(R)-3-CARBOXY-2-(HEXANOYLOXY)-N,N,N-TRIMETHYLPROPAN-1-AMINIUM 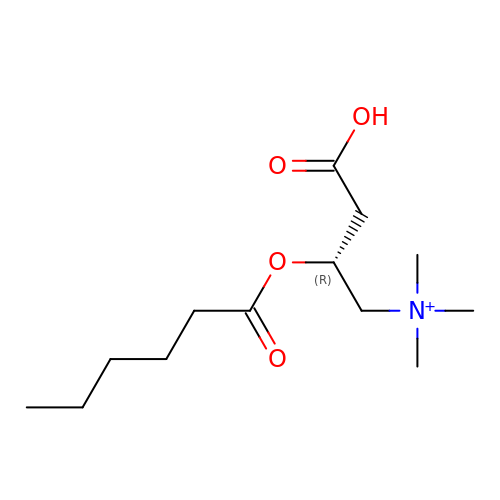| C13 H26 N O4 | VVPRQWTYSNDTEA-LLVKDONJSA-O>HHHHHHMTSERTFIAVKPDGVQRCLVGEIIQRFEKKGYKLVALKMLQPSAEQAQQHYIDLASKPFYKDLVAYFSSGPIVGMVWEGKGVVKGGRVLLGATNPADSLPGTIRGDFAVDVGRNVCHGSDSVDSAKRE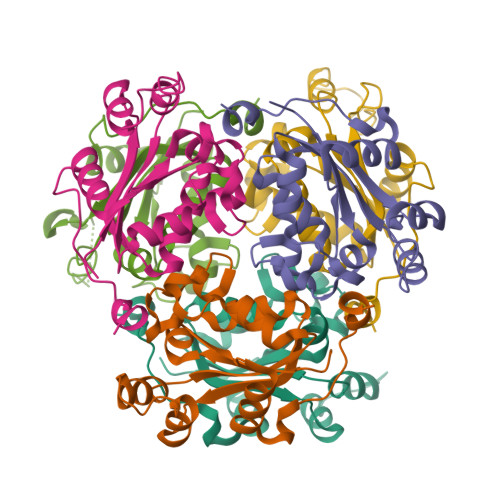IAFWFKPEELVNWTSHSVKQVYE[6x]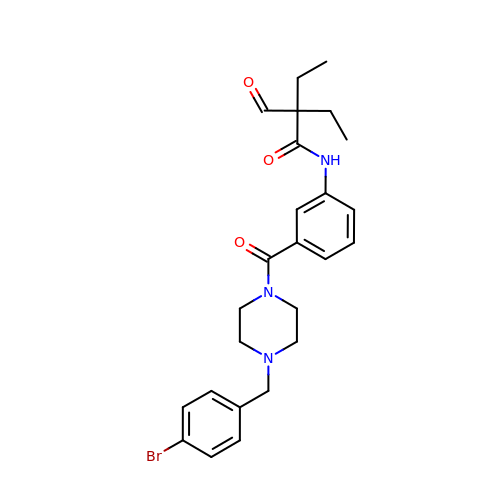~{N}-[3-[4-[(4-bromophenyl)methyl]piperazin-1-yl]carbonylphenyl]-2-ethyl-2-methanoyl-butanamide | C25 H30 Br N3 O3 | OHVWTLFLVCPRSC-UHFFFAOYSA-N>IISRNFPIIGVKEKTFEQLHKKCLEKKVLYVDPEFPPDETSLFYSQKFPIQFVWKRPPEICENPRFIIDGANRTDICQGELGDCWFLAAIACLTLNQHLLFRVIPHDQSFIENYAGIFHFQFWRYGEWVDVVIDDCLPTYNNQLVFTKSNHRNEFWSALLEKAYAKLHGSYEALKGGNTTEAMEDFTGGVAEFFEIRDAPSDMYKI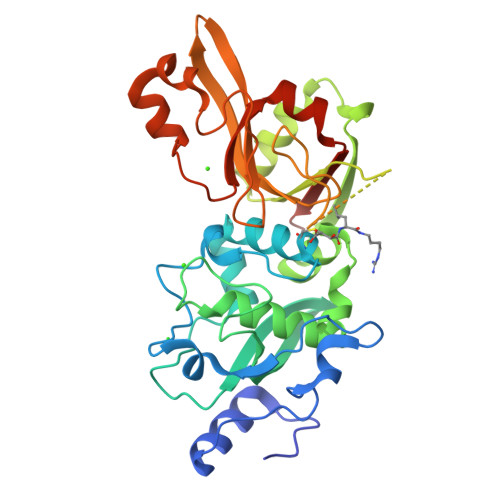MKKAIERGSLMGCSIDDGTNMTYGTSPSGLNMGELIARMVRNMDNSLLQDSDLDPRGSDERPTRTIIPVQYETRMACGLVRGHAYSVTGLDEVPFKGEKVKLVRLRNPWGQVEWNGSWSDRWKDWSFVDKDEKARLQHQVTEDGEFWMSYEDFIYHFTKLEICNLTADLEHHHHHH[4x]>AAIHRTQLWFHGRISREESQRLIGQQGLVDGLFLVRESQRNPQGFV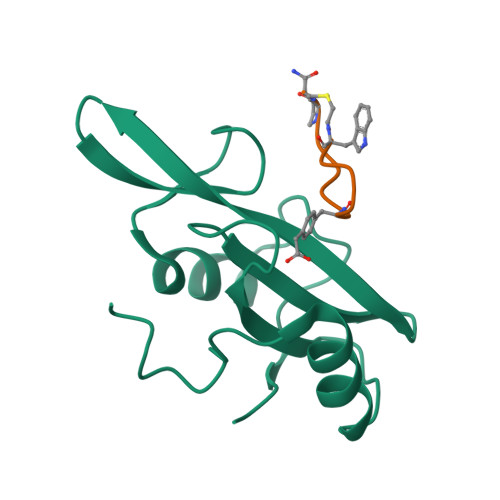LSLCHLQKVKHYLILPSEEEGRLYFSMDDGQTRFTDLLQLVEFHQLNRGILPCLLRHCCTR[2x];>WFEGFDNTFPX[2x]>ALANTFLVKEDSKNVTAYTPFATPITDSKSDLVSLAQLDSSYQIADQTIHNTNLFVLFKSRDVKVKYESSGSNNISFDSTSQGEKPSYVVEFTNSTNIGIKWTMVKKYQLDVPNVSSDMNQVLKNLILEQPLTKYTLNSSLAKEKGKTQREVHLGSGQANQWTSQRNQHDLNNNPSPNASTGFKLTTGNAYRKLSESWPIYEPIDGTKQGKGKDSSGWSSTEENEAKNDAPSVSGGGSSSGTFNKYLNTKQALESIGILFDDQTPRNVITQLYYASTSKLAVTNNHIVVMGNSFLPSMWYWVVERSAQENASNKPTWFANTNLDWGEDKQKQFVENQLGYKETTSTNSHNFHSKSFTQPAYLISGIDSVNDQIIFSGFKAGSVGYDSSSSSSSS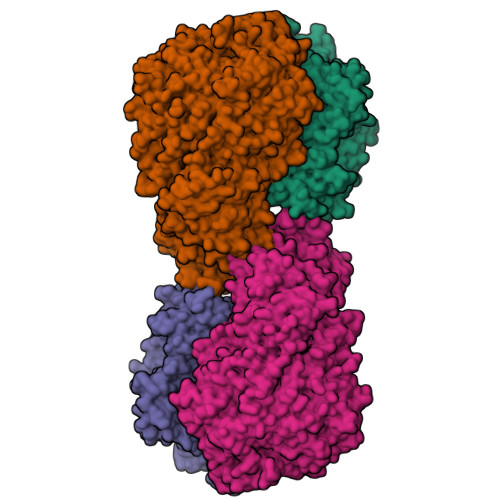SSSSTKDQALAWSTTTSLDSKTGYKDLVTNDTGLNGPINGSFSIQDTFSFVVPYSGNHTNNGTTGPIKTAYPVKKDQKSTVKINSLINATPLNSYGDEGIGVFDALGLNYNFKSNQERLPSRTDQIFVYGIVSPNELRSAKSSADSTGSDTKVNWSNTQSRYLPVPYNYSEGIIDADGFKRPENRGASVTTFSGLKSIAPDGFANSIANFSVGLKAGIDPNPVMSGKKANYGAVVLTRGGVVRLNFNPGNDSLLSTTDNNIAPISFSFTPFTAAESAVDLTTFKEVTYNQESGLWSYIFDSSLKPSHDGKQTPVTDNMGFSVITVSRTGIELNQDQATTTLDVAPSALAVQSGIQSTTQTLTGVLPLSEEFSAVIAKDSDQNKIDIYKNNNGLFEIDTQLSNHHHHHH[4x];>GVITGVGGYFLFNQNKQRSSVSNFAYQPKQLSVKHQQAVDETLTPWTWNNNNFSSLKITGENPGSFGLVRSQNDNLNISSVTKNSSDDNLKYLNAVEKYLDGQQNFAIRRYDNNGRALYDINLAKMENPSTVQRGLNGEPIFDPFKGFGLTGNAPTDWNEIKGKVPVEVVQSPHSPNLYFVLLVPKVALEYHNLNNQVVKESLEVKATQSSFNPTQRLQKDSPVKDSSKQGEKLSETTASSMSSGMATSTRAKALKVEVERGSQSDSLLKNDFAKKPLKHKNSSGEVKLEAEKEFTEAWKPLLTTDQIAREKGMGATVVSFYDAPYSENHTAFGLVDHIDPKKMVENYPPSWKTPKWNHHGIWDYNARNLLLQTTGFFNPRRHPEWFDEGQAKADNTSPGFKVGDTDHKKDGFKKNSSSPIALPFEAYFANIGNMVAIGNSVFIFGGNGHATKMFTTNPLSIGVFRIKYTDNFSKSSVTGWPYAVLFGGLINPQTNGLKDLPLGTNRWFEYVPRMAVSGVKWVGNQLVLAGTLTMGDTATVPRLKYDQLEKHLNLVAQGQGLLREDLQIFTPYGWANRPDIPVGAWLQDEMGSKFGPHYFLNNPDIQDNVNNDTVEALISSYKNTDKLKHVYPYRYSGLYAWQLFNWSNKLTNTPLSANFVNENSYAPNSLFAAILNEDLLTGLSDKIFYGKENEFAENEADRFNQLLSLNPNPNTNWARYLNVVQRFTTGPNLDSSTFDQFLDFLPWIGNGKPFSNSPSPSTSASSSTPLPTFSNINVGVKSMITQHLNKENTRWVFIPNFSPDIWTGAGYRVQSANQKNGIPFEQVKPSNNSTPFDPNSDDNKVTPSGGSSKPTTYPALPNSISPTSDWINALTFTNKNNPQRNQLLLRSLLGTIPVLINKSGDSNDQFNKDSEQKWDKTETNEGNLPGFGEVNGLYNAALLHTYGFFGTNTNSTDPKIGFKADSSSSSSSTLVGSGLNWTSQDVGNLVVINDTSFGFQLGGWFITFTDFIRPRTGYLGITLSSLQDQTIIWADQPWTSFKGSYLDSDGTPKSLWDPTALKSLPNSSTTYDTNPTLSPSFQLYQPNKVKAYQTTNTYNKLIEPVDATSAATNMTSLLKLLTTKNIKAKLGKGTASSQGNNNGGGVSQTINTITTTGNISEGLKEETSIQAETLKKFFDSKQNNKSEIGIGDSTFTKMDGKLTGVVSTPLVNLINGQGATSDSDTEKISFKPGNQIDFNRLFTLPVTELFDPNTMFVYDQYVPLLVNLPSGFDQASIRLKVISYSVENQTLGVRLEFKDPQTQQFIPVLNASSTGPQTVFQPFNQWAHHHHHH[4x]>MVVIGEKFPEVEVKTTHGVIKLPDYFAEQGKWFVLFSHPADCTPVSTTEFYAMQKRVDQFRELGVEPIGLSVDQVFSHIKWMEWIKENLGEEITFPVIADDRGELADKLGMIPSGATITARAVFIVDDKGIIRAIVYYPAEVGRDWDEILRLVKALKVSDEKGVALPHKWPNNELIGDKAIVPPASTVDEVKQREEAK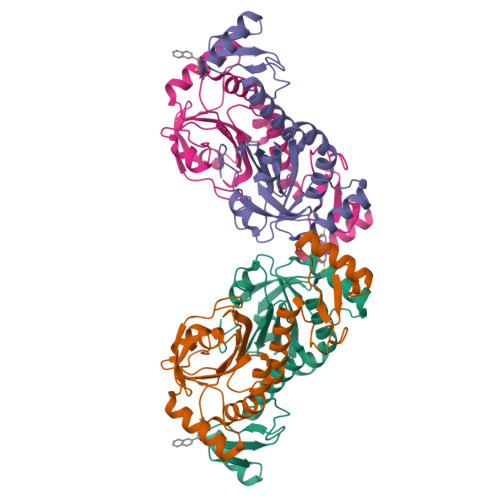AKGEIESYDWWFSYKKLE[2x]> MPTKNRKTDSTSIHASLRHLLQL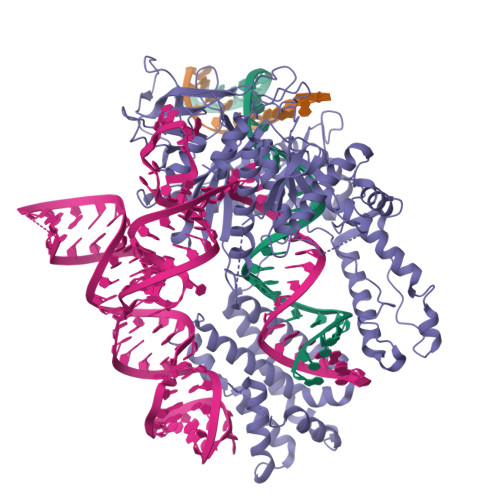GLKRSEAAIPQTITRTAKFKINTAIKPGLIPLLNAQFDAVEGFRRKVLGELEAWWNEDPEAFQKMVKCSMKMKFQGKSSCYAWLYTHFLKGATLAQGLSRDAANSLLDNMGGGLKSFLTRRAHVAEEIRKRYDQNLGDWDDGLKDLAAEHGLELPPPPPRVNFEKLTAQEIEKYNDWVGRTRAWGNLLLIQKKKVERRDACLPRYLKGYPGFPGSQRYATASAMAAALAELEQAAREQYGKARARFAKVSAESWAQTVERFAPAPVRAEHGRPEPRTAHQTVSARLAALIAAQPGWQPAQLAEEILAGVLRGAEKLKTHLSKCGSHDRQAVIKLANLYNVAVAFALEPVRVAGDYLSFYAEETPKRKAFGNVRGALHQPSDDTAAIQITGFSINDEGSPNYNGLLVCKQSGDRLHDEWAFLFCHQPGQVFQLAAEDAKLRGKILTEWLGFGSQGGSRKKAEASAKKMIRRPVWMNEKTPPTILPLAFGVRQGREYLWHFDRNLRTKEGWVLGNGRLLRVMPPGRPHAADFYLTLTLEREAPPLAEVAAEKYIGIARGEAVPAAYAIIDREGRLLAGGKIAEAFRDQQRKTNDEKRELQRTAGGYTKAFRSKERNRARALGGEVTRAIFALSAAHRAPVILANLNSSLATRGGKGTMMSQMQYERMLVALEQKFAEAGLYALPSAPKYRKGDNGFIKLVGPAYTSATCSACGHVHSSDFYEKLADTLEGKCGSSWCVTLPNGEQQQLPDAYTFWLKGKGEQTKSTHERLEELLKGKSVAKLAKTNRRKLVGLLKSRWLPYRATQADFSCVLCGHTMNAAEQGALNIARKFLFRTERGKQAGELTEAERRKMRADWQNWYKEKLRTVWRAPERGDGNG> MPKPINVRVTTMDAE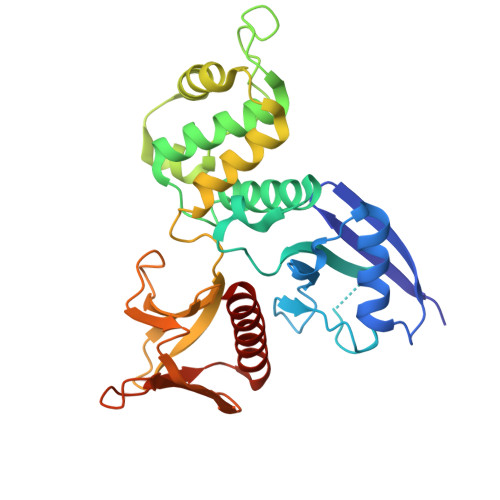LEFAIQPNTTGKQLFDQVVKTIGLREVWYFGLHYVDNKGFPTWLKLDKKVSAQEVRKENPLQFKFRAKFYPEDVAEELIQDITQKLFFLQVKEGILSDEIYCPPETAVLLGSYAVQAKFGDYNKEVHKSGYLSSERLIPQRVMDQHKLTRDQWEDRIQVWHAEHRGMLKDNAMLEYLKIAQDLEMYGINYFEIKNKKGTDLWLGVDALGLNIYEKDDKLTPKIGFPWSEIRNISFNDKKFVIKPIDKKAPDFVFYAPRLRINKRILQLCMGNHELYMRRRK2-(4-AMINO-PHENYL)-5-HYDROXYMETHYL-PYRROLIDINE-3,4-DIOL 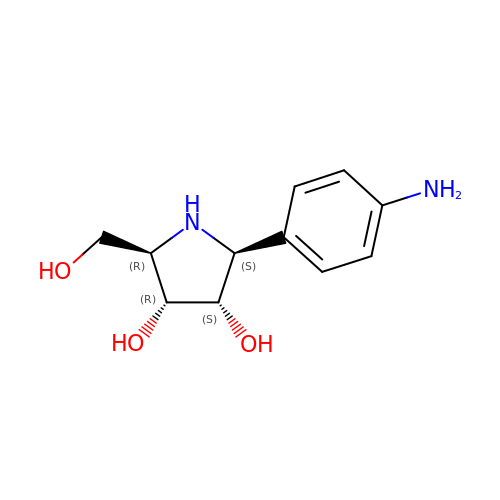| C11 H16 N2 O3 | SQENVZNKXLCDLF-YTWAJWBKSA-N> MHHHHHHDDDDKRTLPGEGTQVHPRAPLLQILKVAGAQEEVFTVKEVMHYLGQYIMMKQLYDKQRQHIVHCHDDPLGELLEV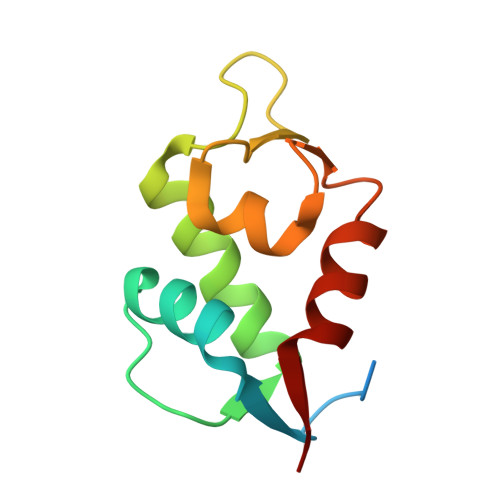GSFSVKNPSPLYEMLKRNLVIL> MTESQSYETRQARPAGQSL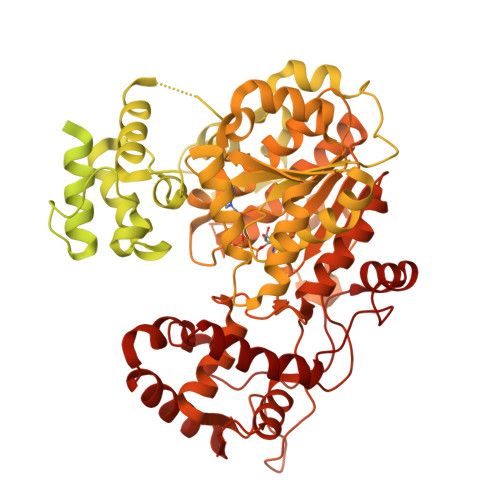AERVARLVAIDPQAAAAVPDKAVAERATQQGLRLAQRIEAFLSGYGDRPALAQRAFEITKDPITGRAVATLLPKFETVSYRELLERSHAIASELANHAEAPVKAGEFIATIGFTSTDYTSLDIAGVLLGLTSVPLQTGATTDTLKAIAEETAPAVFGASVEHLDNAVTTALATPSVRRLLVFDYRQGVDEDREAVEAARSRLAEAGSAVLVDTLDEVIARGRALPRVALPPATDAGDDSLSLLIYTSGSTGTPKGAMYPERNVAQFWGGIWHNAFDDGDSAPDVPDIMVNFMPLSHVAGRIGLMGTLSSGGTTYFIAKSDLSTFFEDYSLARPTKLFFVPRICEMIYQHYQSELDRIGAADGSPQAEAIKTELREKLLGGRVLTAGSGSAPMSPELTAFIESVLQVHLVDGYGSTEAGPVWRDRKLVKPPVTEHKLIDVPELGYFSTDSPYPRGELAIKTQTILPGYYKRPETTAEVFDEDGFYLTGDVVAEVAPEEFVYVDRRKNVLKLSQGEFVALSKLEAAYGTSPLVRQISVYGSSQRSYLLAVVVPTPEALAKYGDGEAVKSALGDSLQKIAREEGLQSYEVPRDFIIETDPFTIENGILSDAGKTLRPKVKARYGERLEALYAQLAETQAGELRSIRVGAGERPVIETVQRAAAALLGASAAEVDPEAHFSDLGGDSLSALTYSNFLHEIFQVEVPVSVIVSAANNLRSVAAHIEKERSSGSDRPTFASVHGAGATTIRASDLKLEKFLDAQTLAAAPSLPRPASEVRTVLLTGSNGWLGRFLALAWLERLVPQGGKVVVIVRGKDDKAAKARLDSVFESGDPALLAHYEDLADKGLEVLAGDFSDADLGLRKADWDRLADEVDLIVHSGALVNHVLPYSQLFGPNVVGTAEVAKLALTKRLKPVTYLSTVAVAVGVEPSAFEEDGDIRDVSAVRSIDEGYANGYGNSKWAGEVLLREAYEHAGLPVRVFRSDMILAHRKYTGQLNVPDQFTRLILSLLATGIAPKSFYQLDATGGRQRAHYDGIPVDFTAEAITTLGLAGSDGYHSFDVFNPHHDGVGLDEFVDWLVEAGHPISRVDDYAEWLSRFETSLRGLPEAQRQHSVLPLLHAFAQPAPAIDGSPFQTKNFQSSVQEAKVGAEHDIPHLDKALIVKYAEDIKQLGLL The reduction of substrates by nitrogenase entails multiple cycles of association and dissociation between two component proteins for sequential transfer of electrons. In the transient complex, electrons are transferred from the [4Fe:4S]-cluster of the homodimeric Fe-protein to the MoFe-protein in a reaction requiring adenosine triphosphate (ATP) hydrolysis. The MoFe-protein, an (αβ)2 tetramer, contains two types of unique metal centers per catalytic αβ-unit: the P-cluster [8Fe:7S] and the FeMo-cofactor [7Fe:9S:C:Mo]-R-homocitrate. The P-cluster is the initial electron acceptor with subsequent transfer to the FeMo-cofactor, one of the most elaborate metalloclusters found in nature and the catalytic center of biological nitrogen reduction.

Se, a structural surrogate for S in [Fe:S] clusters, has crystallographic and spectroscopic properties that make it an excellent probe, hence, potential Se containing compounds were investigated. By screening a range of experimental parameters, we found that Se from SeCN- could be incorporated into the FeMo-cofactor by incubating nitrogenase under assay (turnover) conditions with concentrations of SeCN- sufficient to inhibit acetylene reduction. The 1.60 Å resolution crystal structure of Av1 (Av1-Se2B), isolated from assays containing SeCN-, revealed that Se quantitatively replaced belt-S position S2B in the FeMo-cofactor thereby generating the [7Fe:8S:1Se:Mo:C]-R-homocitrate cluster (FeMoSe-cofactor) form of the MoFe-protein. The essentially exclusive substitution of S2B by Se was validated by anomalous difference Fourier maps calculated from data measured at the Se-K edge f’’-peak position of 12,662 eV. At this resolution, no perturbation of the cofactor structure or its environment was detected, reflecting the small increase (3.8%) in the ionic radius of Se relative to S. Except for a low occupancy site (ranging from 0–20% under different conditions) adjacent to the previously identified potential sulfur-binding site (located ~22 Å away from the FeMo-cofactor at the interface of the α and β subunits [Spatzal et al., 2014]), no other Se sites were identified in the anomalous difference Fourier map. Significantly, Av1-Se2B retains acetylene and dinitrogen reduction activity when compared to native Av1, with the difference that the activity time course for Av1-Se2B with acetylene and dinitrogen exhibits a longer initial lag phase than for native Av1. Consequently, the ability to prepare site-specifically labeled FeMoSe-cofactor provided the starting point for a structural investigation of the active site during substrate (acetylene) turnover. (A) Side view of FeMoSe-cofactor ([7Fe:8S:1Se:Mo:C]-R-homocitrate) in Av1-Se2B at a resolution of 1.60 Å, highlighting the S2B replacement by Se. The 2Fo-Fc density at the Se2B site is significantly increased compared to the S5A and S3A sites.

>[2x]MTGMSREEVESLIQEVLEVYPEKARKDRNKHLAVNDPAVTQSKKCIISNKKSQPGLMTIRGCAYAGSKGVVWGPIKDMIHISHGPVGCGQYSRAGRRNYYIGTTGVNAFVTMNFTSDFQEKDIVFGGDKKLAKLIDEVETLFPLNKGISVQSECPIGLIGDDIESVSKVKGAELSKTIVPVRCEGFRGVSQSLGHHIANDAVRDWVLGKRDEDTTFASTPYDVAIIGDYNIGGDAWSSRILLEEMGLRCVAQWSGDGSISEIELTPKVKLNLVHCYRSMNYISRHMEEKYGIPWMEYNFFGPTKTIESLRAIAAKFDESIQKKCEEVIAKYKPEWEAVVAKYRPRLEGKRVMLYIGGLRPRHVIGAYEDLGMEVVGTGYEFAHNDDYDRTMKEMGDSTLLYDDVTGYEFEEFVKRIKPDLIGSGIKEKFIFQKMGIPFRQMHSWDYSGPYHGFDGFAIFARDMDMTLNNPCWKKLQAPWEASEGAEKVAASA;>MSQQVDKIKASYPLFLDQDYKDMLAKKRDGFEEKYPQDKIDEVFQWTTTKEYQELNFQREALTVNPAKACQPLGAVLCALGFEKTMPYVHGSQGCVAYFRSYFNRHFREPVSCVSDSMTEDAAVFGGQQNMKDGLQNCKATYKPDMIAVSTTCMAEVIGDDLNAFINNSKKEGFIPDEFPVPFAHTPSFVGSHVTGWDNMFEGIARYFTLKSMDDKVVGSNKKINIVPGFETYLGNFRVIKRMLSEMGVGYSLLSDPEEVLDTPADGQFRMYAGGTTQEEMKDAPNALNTVLLQPWHLEKTKKFVEGTWKHEVPKLNIPMGLDWTDEFLMKVSEISGQPIPASLTKERGRLVDMMTDSHTWLHGKRFALWGDPDFVMGLVKFLLELGCEPVHILCHNGNKRWKKAVDAILAASPYGKNATVYIGKDLWHLRSLVFTDKPDFMIGNSYGKFIQRDTLHKGKEFEVPLIRIGFPIFDRHHLHRSTTLGYEGAMQILTTLVNSILERLDEETRGMQATDYNHDLVR[2x]> MKRQWALEDFEIGRPLGKGKFGNVYLAREKQSKFILALKVLFKAQLEKAGVEHQLRREVEIQSHLRHPNILRLYGYFHDATRVYLILEYAPLGTVYRELQKLSKFDEQRTATYITELANALSYCHSKRVIHRDIKPENLLLGSAGELKIADFGWSVHAPSSRRTDLCGTLDYLPPEMIEGRMHDEKVDLWSLGVLCYEFLVGKPPFEANTYQETYKRISRVEFTF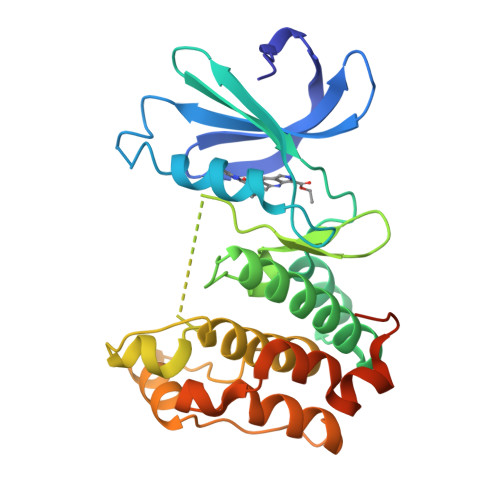PDFVTEGARDLISRLLKHNPSQRPMLREVLEHPWITANSSKPSNCQNKESAAAALEHHHHHH> GSHMNEVTLLDSRSVQGELGWIASPLEGGWEEVSIMDEKNT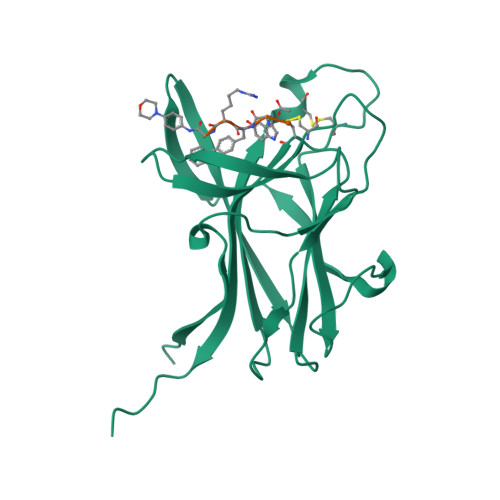PIRTYQVCNVMEPSQNNWLRTDWITREGAQRVYIEIKFTLRDCNSLPGVMGTCKETFNLYYYESDNDKERFIRENQFVKIDTIAADESFTQVDIGDRIMKLNTEIRDVGPLSKKGFYLAFQDVGACIALVSVRVFYKKAPLTVR>MAPIAGKKAKRGILERLNAGEVVIGDGGFVFALEKRGYVKAGPWTPEAAVEHPEAVRQLHREFLRAGSNVMQTFTFYASEDKLENRGNYVAEKISGQKVNEAACDIARQVADEGDALVAGGVSQTPSYLSCKSETEVKKIFHQQLEVFMKKNVDFLIAEYFEHVEEAVWAVEALKTSGKPIAATMCIGPEGDLHGVSPGECAVRLVKAGAAIVGVNCHFDPSTSLQTIKLMKEGLEAARLKAYLMSQPLAYHTPDCGKQGFIDLPEFPFGLEPRVATRWDIQKYAREAYNLGVRYIGGCCGFEPYHIRAIAEELAPERGFLPPASEKHGSWGSGLDMHTKPWIRARARKEYWQNLRIASGRPYNPSMSKP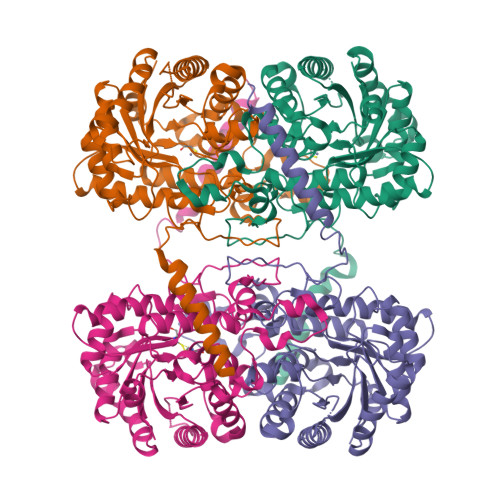DAWGVTKGAAELMQQKEATTEQQLRALFEKQKFKSAQ[4x]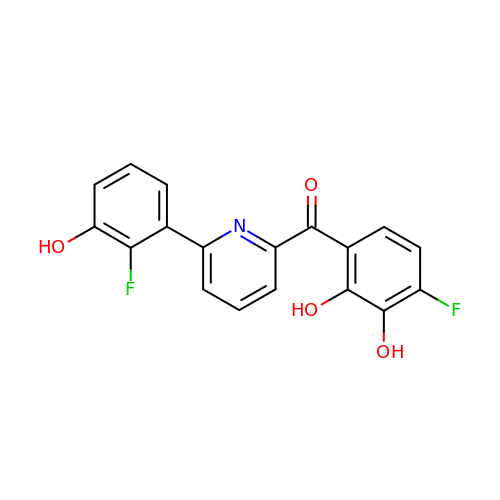[4-fluoranyl-2,3-bis(oxidanyl)phenyl]-[6-(2-fluoranyl-3-oxidanyl-phenyl)pyridin-2-yl]methanone | C18 H11 F2 N O4 | ACRZIJAMHSRKJJ-UHFFFAOYSA-N>GHMTHSAYVYQLKAVPDIFDEISQRFPDRVALIFDQRKITYRELAEQCSALAAVLQNNCLIKGDIVAIKIERSPELYIFMLALMKIGAVMVPVNSNSPERYIGEVLSAAGARYLISDDVTSVPGGAWHVLSSRTLIQNCTQQRSGNYPVLSADDPALILMTSGSTGKPKSVLIAHRGIARLGLPVPALGNSERDCYLQIADISFAASANEIWMALLTGACLTIAPPGLPDLMALARQIESDNVTMLFLSGGLFRLFVEVSVETLHIPDCVVVSGDFVNPRLFSVAVQAGKAKIFNGLGCTENSAISSLYHIQSAAALSSESPVPVGTPLPLVEMVVFNERLQPCTCGEYGELFIAGAGVALGYSDPQLTAERFITIPYQGTDMLFYRTDDRATYDQDRNIVLVGRGNHICKIRGFRINIAGIEHLLRLHHAVEDVLIVVEETPDEPRLHACYVTQDDGLSVADLKNHLAMHAPAWMIPEKFSRLAVLPMTANGKKDRLRLKNSLLEQVASMDNVEQQLLSIWQAIIHSEAINPQENLLDQGGNSLHFIKLASMVSKTFNL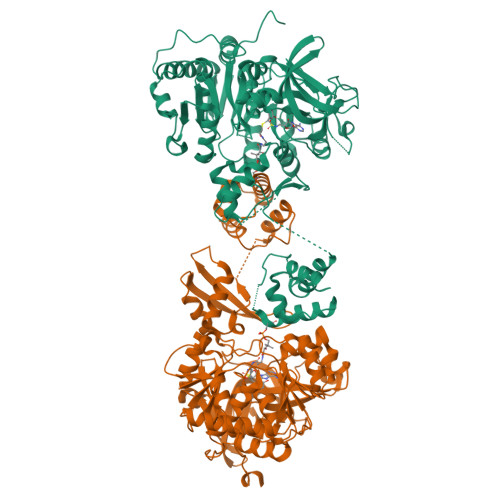AVSPADIFTAGTIAALAQTIRQRQKL[4x]> GSGSGSGMSWIKEGELSLWERFCANIIKAGPMPKHIAFIMDGNRRYAKKCQVERQEGHSQGFNKLAETLRWCLNLGILEVTVYAFSIENFKRSKSEVDGLMDLARQKFSRLMEEKEKLQKHGVCIRVLGDLHLLPLDLQELIAQAVQATKNYNKCFLNVCFAYTSRHEISNAVREMAWGVEQGLLDPSDISESLLDKCLYTNRSPHPDILIRTSGEVRLSDFLLWQTSHSCLVFQPVLWPEYTFWNLFEAILQFQMNHSVLQKAR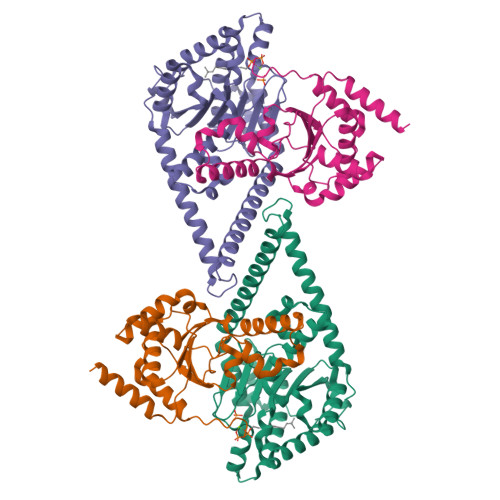DMYAEERKRQQLERDQATVTEQLLREGLQASGDAQLRRTRLHKLSARREERVQGFLQALELKRADWLARLGTASA;> GSGSGSGRGGSCLAAAHHRMRWRADGRSLEKLPVHMGLVITEVEQEPSFSDIASLVVWCMAVGISYISVYDHQGIFKRNNSRLMDEILKQQQELLGLDCSKDKDDQVLNCHLAVKVLSPEDGKADIVRAAQDFCQLVAQKQKRPTDLDVDTLASLLSSNGCPDPDLVLKFGPVDSTLGFLPWHIRLTEIVSLPSHLNISYEDFFSALRQYAACEQRLGK The transport of the CagA effector into gastric epithelial cells by the Cag Type IV secretion system (Cag T4SS) of Helicobacter pylori (H. pylori) is critical for pathogenesis. CagA is recruited to Cag T4SS by the Cagβ ATPase. CagZ, a unique protein in H. pylori, regulates Cagβ-mediated CagA transport, but the underlying mechanisms remain unclear. Our structural and biochemical data together show that Cagβ functions as a dynamic hexameric assembly.

We crystallized the soluble region of Cagβ (residues 166–748; referred to as Cagβ1) and collected an X-ray diffraction dataset to 2.8 Å resolution. Molecular replacement using this model found all six protomers in the asymmetric unit of the crystal, which together form a pseudo-6-fold symmetric hexameric assembly. The protomer of Cagβ shows a 3-layered overall architecture similar to TrwB. Residues 631–658, an extended segment between two α-helices in the NBD, form two long anti-parallel β-strands that stray away from the NBD and constitute the bottom layer of the 3-layered Cagβ. These extended β-strands from the six subunits together form a 12-stranded β-barrel, contributing to the hexameric assembly. As in other hexameric ATPases, the NBD makes a major contribution to the inter-subunit interface for the formation of the hexamer, resulting in the placement of the ATP-binding site at the inter-subunit interface. The six subunits in the Cagβ hexamer are not related by a perfect 6-fold symmetry. The asymmetry in the Cagβ hexamer structure may reflect its intrinsic dynamic nature and ability to carry out sequential translocation of CagA through the channel at the middle of the hexamer. The central channel in the Cagβ hexamer runs continuously from the cytosol end to the membrane-proximal end, spanning a distance of ~100 Å. Strong density is present near the Walker A and B motifs in the structure, which was assigned to a sulfate group from the crystallization buffer, mimicking the binding of ATP to the nucleotide-binding site. Our structure of the Cagβ hexamer shows that no arginine residue from the neighboring subunit is present near the ATP-binding site of the NBD, suggesting R241 in the Walker A motif may fulfill the role of the arginine finger in cis.

>[6x]GTSSMADIGSKYLTRTRDIGANKKVDDLFGSASWETEEKMIKAKLITPNNKKRAFDKREVIVGRRGLGDFIAYAGQAFIGLIAPTRSGKGVGFIMPNMINYPQNIVVFDPKADTMETCGKIREKRFNQKVFIYEPFSLKTHRFNPFAYVDFGNDVVLTEDILSQIDTRLKGHGMVASGGDFSTQIFGLAKLVFPERPNEKDPFFSNQARNLFVINCNIYRDLMWTKKGLEFVKRKKIIMPETPTMFFIGSMASGINLIDEDTNMEKVVSLMEFFGGEEDKSGDNLRVLSPATRNMWNSFKTMGGARETYSSVQGVYTSAFAPYNNAMIRNFTSANDFDFRRLRIDEVSIGVIANPKESTIVGPILELFFNVMIYSNLILPIHDPQCKRSCLMLMDEFTLCGYLETFVKAVGIMAEYNMRPAFVFQSKAQLENDPPLGYGRNGAKTILDNLSLNMYYGINNDNYYEHFEKLSKVLGKYTRQDVSRSIDDNTGKTNTSISNKERFLMTPDELMTMGDELIILENTLKPIKCHKALYYDDPFFTDELIKVSPSLSKKYKLGKVPNQATFYDDLQAAKTRGELSYDKSLVPVGSSEL>SATTPPGDLEQPELEARVKEIIEVDGYQFRDLNDNGELDPYEDWRLPTPERVADLVGQMSLVEKSGLMLINTLNAACDPQTGEFGVLPAQADNYINTQHMHRFVFRNVVDVRAEGVECTGTGTPVVSPAEAATFTNAVQEMSEATRLGIPSLFKSNARNHIDPDARVGINEAAGAFSAFPKEAGIAAAALGEQARRTGEATTGDMSVVADFADVMGEEWASIGLRGMYGYMADLSTEPRWYRTHETFTEDAYLAAEIMETLVQTLQGEELTDNGLALSPQTRVALTLKHFPGGGPQELGLDPHYAFGKAQVYPAGRFEEHFLPFQAAIDAGVSSIMPYYGVPVDVPVVGGEPGETYPHTGFAFSDSIVNGLLRDQLGFTGYVNSDTGIINDRAWGLEGNTVPERVAAAINGGTDTLSGFSDVSVITDLYEADLISEERIDLAAERLLEPLFDMGLFENPYVDPDVATATVGADDHRAVGLDLQRKSLVLLQNEETDEGPVLPLKEGGDVYILGDFTEETVESYGYEVTNGNVAEGEERPSAAGSDYVLISMTAKTNAGDYVSDDPSLGLNPDHGTNPSVIIGDDGEPLPGLDGQSLWGAADVCVHKEGHEENPSCTDNRLRFGGAYPWESSILDFTGMEAAESWEVVPSLETIQEVMAEVEDPSKVILHVYFRQPYVLDEESGLRDAGAILAGFGMTDTALMDVLTGAYAPQGKLPFALAGTREAIIEQDSD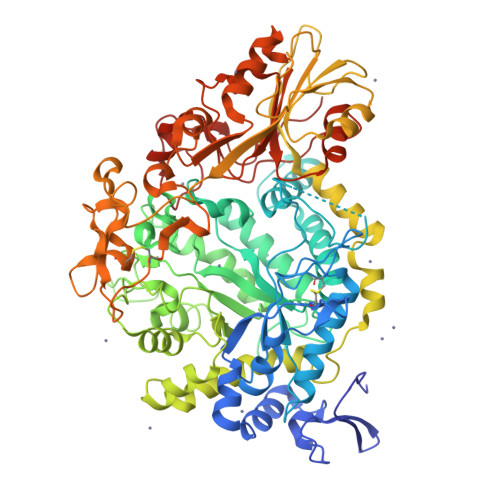RPGYDETEDGALYPFGYGLTYEDDTEE[2x]> 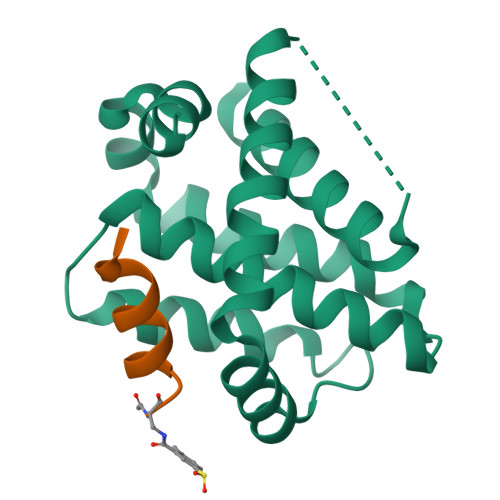GSHMDELYRQSLEIISRYLREQATGAKDTKPMGRSGATSRKALETLRRVGDGVQRNHETAFQGMLRKLDIKNEDDVKSLSRVMIHVFSDGVTNWGRIVTLISFGAFVAKHLKTINQESCIEPLAESITDVLVRTKRDWLVKQRGWDGFVEFFHVED;> XIAEQLRRIGDRF> NDKLVELSKSDDNWVMPGKNYDSNNFSDLKQINKGNVKQLRPAWTFSTG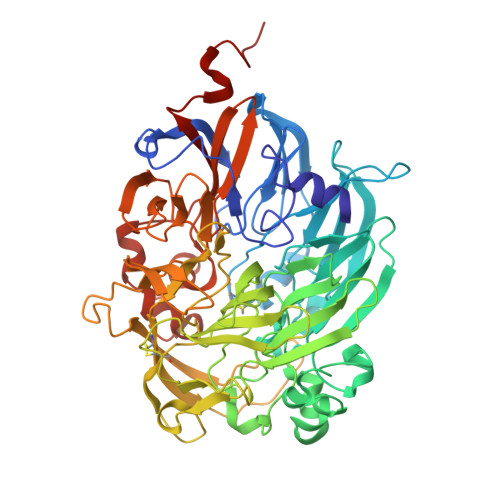LLNGHEGAPLVVDGKMYIHTSFPNNTFALGLDDPGTILWQDKPKQNPAARAVACCDLVNRGLAYWPGDGKTPALILKTQLDGNVAALNAETGETVWKVENSDIKVGSTLTIAPYVVKDKVIIGSSGAELGVRGYLTAYDVKTGEQVWRAYATGPDKDLLLASDFNIKNPHYGQKGLGTGTWEGDAWKIGGGTNWGWYAYDPGTNLIYFGTGNPAPWNETMRPGDNKWTMTIFGRDADTGEAKFGYQKTPHDEWEYAGVNVMMLSEQKDKDGKARKLLTHPDRNGIVYTLDRTDGALVSANKLDDTVNVFKSVDLKTGQPVRDPEYGTRMDHLAKDICPSAMGYHNQGHDSYDPKRELFFMGINHICMDWEPFMLPYRAGQFFVGATLNMYPGPKGDRQNYEGLGQIKAYNAITGDYKWEKMERFAVWGGTMATAGDLVFYGTLDGYLKARDSDTGDLLWKFKIPSGAIGYPMTYTHKGTQYVAIYYGVGGWPGVGLVFDLADPTAGLGAVGAFKKLANYTQMGGGVVVFSLDGKGPYDDPNVGEWKSAAK> LPDYVDWRSSGAVVDIKDQGQCGSCWAFSTIAAVEGINKIATGDLISLSEQELVDCGRTQNTRGCDGGFMTDGFQFIINNGGINTEANYPYTAEEGQCNLDLQQEKYVSIDTYENVPYNNEWALQTAVAYQPVSVALEAAGYNFQHYSSGIFTGPCGTAVDHAVTIVGY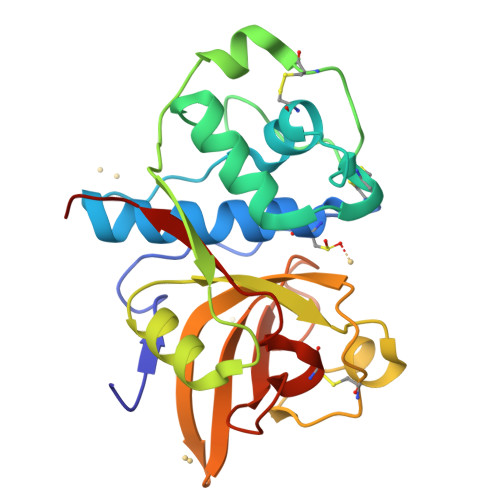GTEGGIDYWIVKNSWGTTWGEEGYMRIQRNVGGVGQCGIAKKASYPVKYYN> FDVGDEYEIIETIGNGAYGVVSSARRRLTGQQVAIKKIPNAFDVVTNAKRTLRELKILKHFKHDNIIAIKDILRPTVPYGEFKSVYVVLDLMESDLHQIIHSSQPLTLEHVRYFLYQLLRGLKYMHS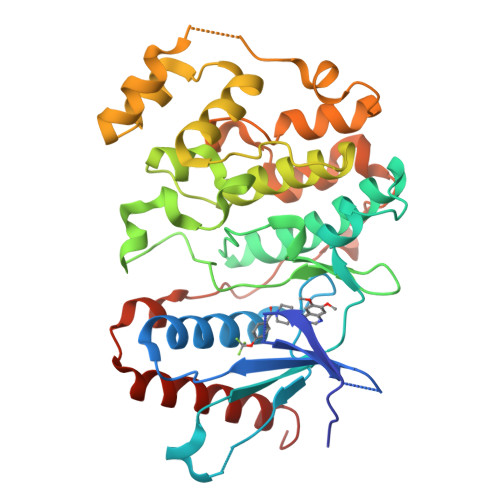AQVIHRDLKPSNLLVNENCELKIGDFGMARGLCTSPAEHQYFMTEYVATRWYRAPELMLSLHEYTQAIDLWSVGCIFGEMLARRQLFPGKNYVHQLQLIMMVLGTPSPAVIQAVGAERVRAYIQSLPPRQPVPWETVYPGADRQALSLLGRMLRFEPSARISAAAALRHPFLAKYHDPDDEPDCAPPFDFAFDREALTRERIKEAIVAEIEDFHARREGI>[2x]AAQGSAGSMLKPQQTTTRDLISLDGLWKFALASDDNNTQPWTSQLKTSLECPVPASYNDIFADSKIHDHVGWVYYQRDVIVPKGWSEERYLVRCEAATHHGRIYVNGNLVADHVGGYTPFEADITDLVAAGEQFRLTIAVDNELTYQTIPPGKVEILEATGKKVQTYQHDFYNYAGLARSVWLYSVPQQHIQDITVRTDVQGTTGLIDYNVVASTTQGTIQVAVIDEDGTTVATSSGSNGTIHIPSVHLWQPGAAYLYQLHASIIDSSKKTIDTYKLATGIRTVKVQGTQFLINDKPFYFTGFGKHEDTNIRGKGHDDAYMVHD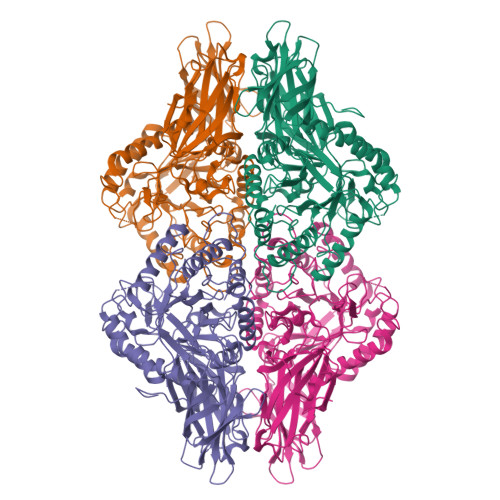FQLLHWMGANSFRTSHYPYAEEVMEYADRQGIVVIDETPAVGLAFSIGAGAQTSNPPATFSPDRINNKTREAHAQAIRELIHRDKNHPSVVMWSIANEPASNEDGAREYFAPLPKLARQLDPTRPVTFANVGLATYKADRIADLFDVLCLNRYFGWYTQTAELDEAEAALEEELRGWTEKYDKPIVMTEYGADTVAGLHSVMVTPWSEEFQVEMLDMYHRVFDRFEAMAGEQVWNFADFQTAVGVSRVDGNKKGVFTRDRKPKAAAHLLRKRWTNLHNGTAEGGKTFQ>MHHHHHHQIGWRREGIKYRRNELFLDVLESVNLLMSPQGQVLSAHVSGRVVMKSYLSGMPECKFGMNDKIVIEKQGKGTADETSKSGKQSIAIDDCTFHQCVRLSKFDSERSISFIPPDGEFELMRYRTTKDIILPFRVIPLVREVGRTKLEVKVVIKSNFKPSLLAQKIEVRIPTPLNTSGVQVICMKG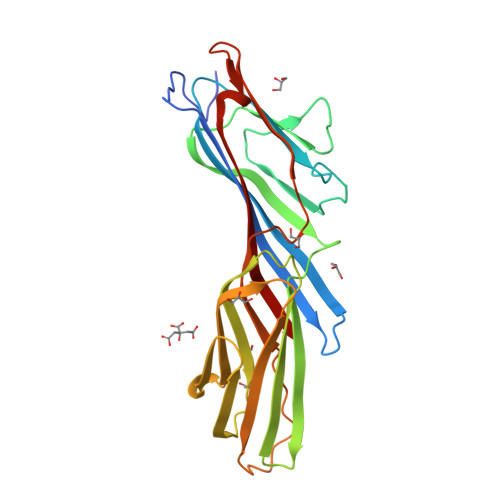KAKYKASENAIVWKIKRMAGMKESQISAEIELLPTNDKKKWARPPISMNFEVPFAPSGLKVRYLKVFEPKLNYSDHDVIKWVRYIGRSGIYETRC[2x]>MDFVS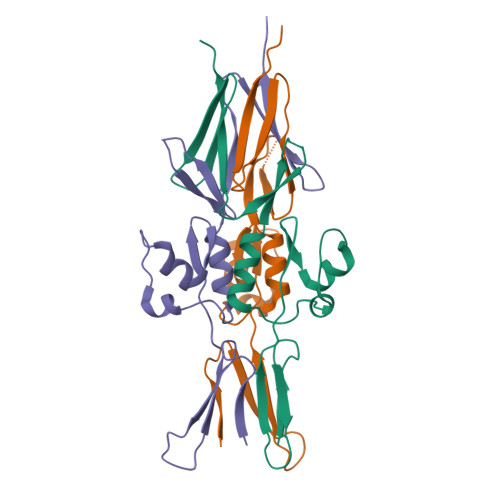GDKDTTSVTVESKDNGKRTEVKIGAKTSVIKDHNGKLFTGKELKDANNNGVTVTETDGKDEGNGLVTAKAVIDAVNKAGWRVKTTGANGQNDDFATVASGTNVTFADGNGTTAEVTKANDGSITVKYNVKVADGLKLDLEHHHHHH[9x]CDT is a member of the Iota family of protein toxins which also consists of two homologous toxins produced by Clostridium perfringens (the Iota toxin) and Clostridium spiroforme (C. spiroforme Transferase, CST). All three Iota toxin family members are assembled from two polypeptide chains termed the “A” subunit (CDTa, Ia, and CSTa) and “B”, subunit (CDTb, Ib, and CSTb). All three B subunits are presumed to contain five domains that are involved in regulation (D1), oligomerization (D2 and D3), and host recognition (D3’ and D4). Once proteolyzed, the mature form of CDTb forms a large heptameric, soluble structure referred to as the prepore which binds one molecule of CDTa to generate the toxic moiety, CDT.

Further classification and refinement of the CDTb dimer led to a map with a final resolution of 3.56 Å, with local resolutions consistent throughout much of the map (S3A). Modeling of the CDTb dimer resulted in the assignment of two chains that we call ‘Chain A’ and ‘Chain B’, both of which were observed in a prepore-like configuration with three additional nodes of density that we modeled as calcium ions in agreement with previous studies. The modeled portions of the two chains are nearly identical in structure with a low backbone RMSD (0.945 Å), though differences in the residues that could be modeled do exist. The receptor binding domain (D4) was not observed in either chain in contrast to previous structures though additional density is present, indicating the D4 domain remains flexible during toxin assembly. Chains A and B are arranged in positions and orientations that are similar to that observed in the prepore structure, though Chain B is rotated ~40° about the central pseudosymmetric axis in the dimeric intermediate, as opposed to ~51° in the structure of the prepore, illustrating structural plasticity at the dimeric interface during assembly. The surface formed between Chains A and B accounts for ~1,200 Å2 of buried surface area and relies primarily on structures formed by residues 411–423, 477–484, 504–513, and 534–541 from Chain A and residues 237–240, 278–290, 427–434, 439–451, and 490–498 from Chain B for assembly. All residues contained within this interface are also observed in the structure of the symmetric heptamer, reconstructed from the same dataset. One site of interaction comprised of structures formed by residues 384–388 and 456–463 of Chain A and residues 314–318 and 451–454 of Chain B was observed in the previously defined structure of the CDTb prepore but is not found to interface in the oligomeric intermediate suggesting it is only engaged in the fully formed toxin.

>[2x]MKIQMRNKKVLSFLTLTAIVSQALVYPVYAQTSTSNHSNKKKEIVNEDILPNNGLMGYYFTDEHFKDLKLMAPIKDGNLKFEEKKVDKLLDKDKSDVKSIRWTGRIIPSKDGEYTLSTDRDDVLMQVNTESTISNTLKVNMKKGKEYKVRIELQDKNLGSIDNLSSPNLYWELDGMKKIIPEENLFLRDYSNIEKDDPFIPNNNFFDPKLMSDWEDEDLDTDNDNIPDSYERNGYTIKDLIAVKWEDSFAEQGYKKYVSNYLESNTAGDPYTDYEKASGSFDKAIKTEARDPLVAAYPIVGVGMEKLIISTNEHASTDQGKTVSRATTNSKTESNTAGVSVNVGYQNGFTANVTTNYSHTTDNSTAVQDSNGESWNTGLSINKGESAYINANVRYYNTGTAPMYKVTPTTNLVLDGDTLSTIKAQENQIGNNLSPGDTYPKKGLSPLALNTMDQFSSRLIPINYDQLKKLDAGKQIKLETTQVSGNFGTKNSSGQIVTEGNSWSDYISQIDSISASIILDTENESYERRVTAKNLQDPEDKTPELTIGEAIEKAFGATKKDGLLYFNDIPIDESCVELIFDDNTANKIKDSLKTLSDKKIYNVKLERGMNILIKTPTYFTNFDDYNNYPSTWSNVNTTNQDGLQGSANKLNGETKIKIPMSELKPYKRYVFSGYSKDPLTSNSIIVKIKAKEEKTDYLVPEQGYTKFSYEFETTEKDSSNIEITLIGSGTTYLDNLSITELNSTPEILDEPEVKIPTDQEIMDAHKIYFADLNFNPSTGNTYINGMYFAPTQTNKEALDYIQKYRVEATLQYSGFKDIGTKDKEMRNYLGDPNQPKTNYVNLRSYFTGGENIMTYKKLRIYAITPDDRELLVLSVD>HHHHHHGSMQILLANPRGFCAGVDRAISIVENALAIYGAPIYVRHEVVHNRYVVDSLRERGAIFIEQISEVPDGAILIFSAHGVSQAVRNEAKSRDLTVFDATCPLVTKVHMEVARASRRGEESILIGHAGHPEVEGTMGQYSNPEGGMYLVESPDDVWKLTVKNEEKLSFMTQTTLSVDDTSDVIDALRKRFPKIVGPRKDDICYATTNRQEAVRALAEQAEVVLVVGSKNSSNSNRLAELAQRMGKRAFLIDDA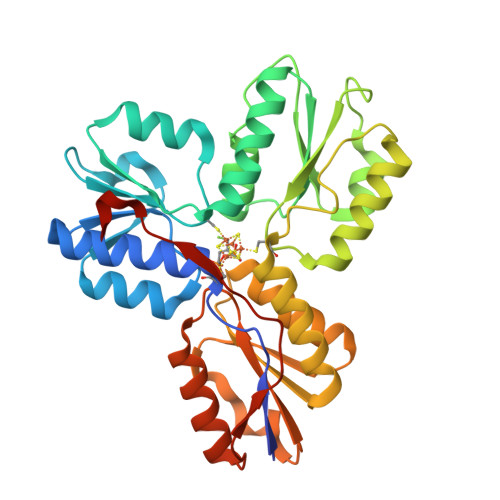KDIQEEWVKEVKCVGVTAGASAPDILVQNVVARLQQLGGGEAIPLEGREENIVFEVPKELRVDIREV[2x]>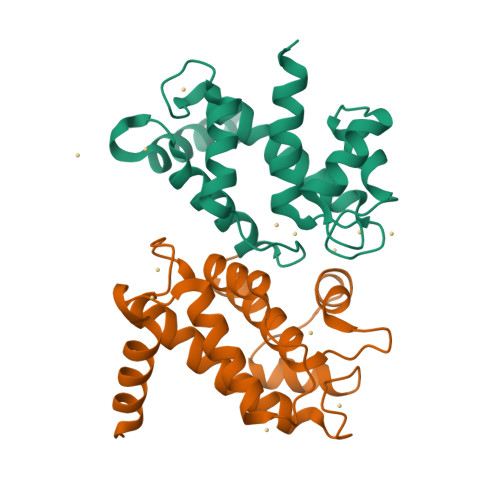[2x]NIEANESEEERQFRKLFVQLAGDDMEVSATELMNILNKVVTRHPDLKTDGFGIDTCRSMVAVMDSDTTGKLGFEEFKYLWNNIKKWQGIYKRFDTDRSGTIGSNELPGAFEAAGFHLNQHIYSMIIRRYSDETGNMDFDNFISCLVRLDAMFRAFRSLD>SMKEPSQQRVKRWGFGMDEALKDPVGREQFLKFLESEFSSENLRFWLAVEDLKKRPIKEVPSRVQEIWQEFLAPGAPSAINLDSKSYDKTTHNVKEPGRYTFEDAQEHIYKLMKSDSYPRFIRSSAYQELLQAKKKSGNSMDRRTS[2x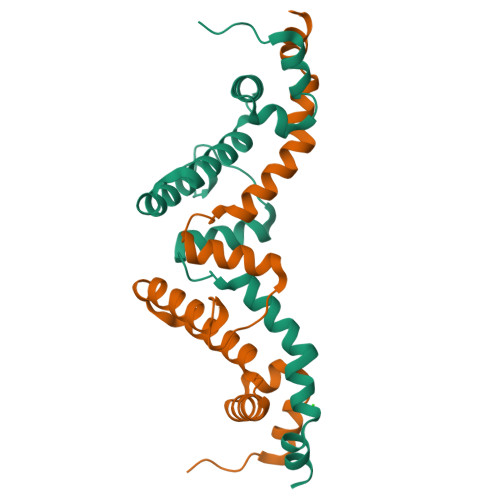]(3S,6S)-3-benzyl-6-(4-hydroxybenzyl)piperazine-2,5-dione 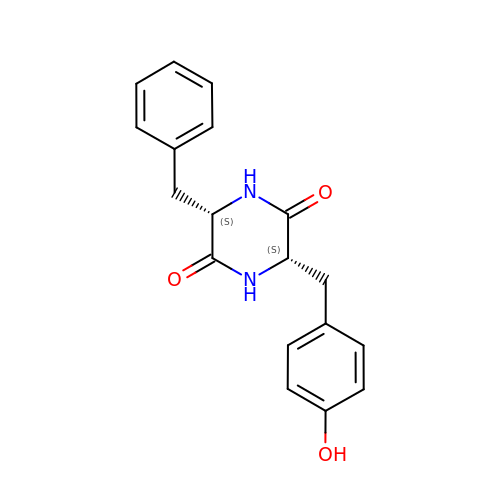| C18 H18 N2 O3 | GRWVBLRIPRGGPD-HOTGVXAUSA-N> GIEDLITEVAQGALTLSLPKQQDSLPDTKASGPAHSKEVPALTAVETG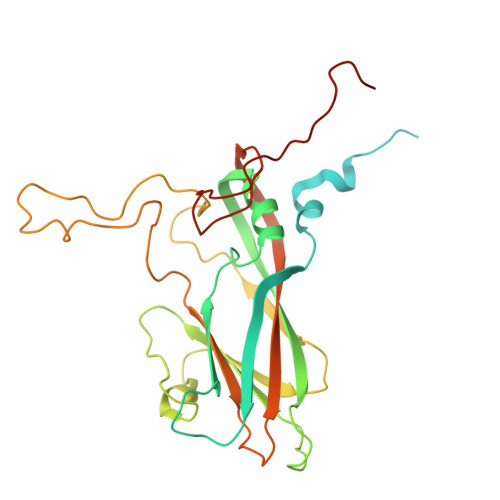ATNPLVPSDTVQTRHVIQRRSRSESTIESFFARGACVAIIEVDNEEPTTRAQKLFAMWRITYKDTVQLRRKLEFFTYSRFDMELTFVVTANFTNTNNGHALNQVYQIMYIPPGAPTPKSWDDYTWQTSSNPSIFYTYGAAPARISVPYVGLANAYSHFYDGFAKVPLKTDANDQIGDSLYSAMTVDDFGVLAIRVVNDHNPTKVTSKVRIYMKPKHVRVWCPRPPRAVPYYGPGVDYKDNLNPLSEKGLTTY> ASGDIVLFSGSKHVEFTDWGGTDWPSAYELQPPYQTMPFDLNKNFEIKVDYSGADIVLIFARWEHGSKPQIWAQISPYYVVDGTAVFTKEQIAKAYGSDDF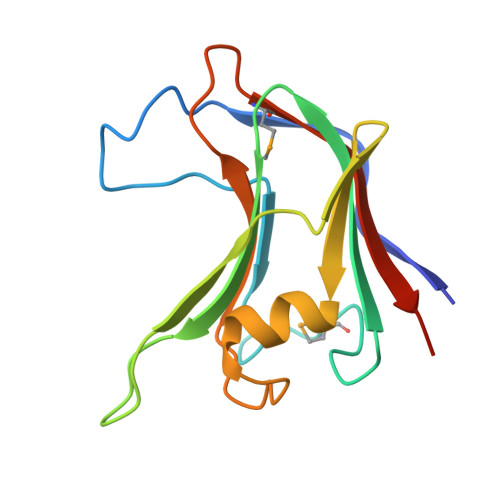SDLDYIGVKPLPSADGMTVTKIVASYTSGSSDD> MPGREILVLHVGQGGNQIGYNFWKTICEEHNIDIRSNQRKSVEEDKVDYKSVFLVEAPDGFHPRALFIDLEPLAVEFLVKEMKLGSFFSEDLMVLSYSGAHNVWSIGYQTGKKLIPVILEKIRDTMPETLQGFLIIHTLGGGTGSGFGSLLTETLKKEFPGKGVLNFSVLPSEVNDVTLAPYNTVLSLNHLSRFSDLVVLFDNTALIRIVKDQLNYPVIKQFSDLNFLIGRVMASITASLRFPGPLNMDLMEMAHNLVALPETKFIIPSVAPLTKEESEMSTELDLVERCFDPTHYMVNCSG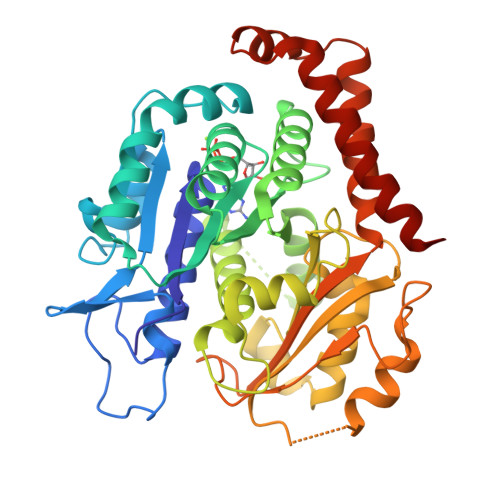QGKTISSVLMFRGNIAIENAFSIMTDIKSNVAFAPGVHPDLGLKYGICESAPVDFDKEVTLLSNNTIISEVFNRVLERFDSLFNRDWYTSDYVNAGTSKSNLKEARDNFDRIIKIYKEIEGSQ L. pneumophila inhibits autophagy by injecting an effector protein called RavZ into the cytoplasm. RavZ functions as a cysteine protease and irreversibly deconjugates mammalian Atg8s from PE to inhibit autophagosome formation. Unlike Atg4 that cleaves the amide bond between terminal glycine and PE, RavZ cleaves the amide bond before glycine. As a consequence, the RavZ-cleaved Atg8 proteins cannot be relipidated, leading to inhibition of autophagy.

Next, we solved the structures of two RavZ fragments, 1–487 and 20–502. Crystal structures of the fragments are essentially identical, solved in space group I422. RavZ structures of both fragments are resolved from residues 47 to 433 and 48 to 432, respectively, whereas the missing regions at the N- and C-termini (residues 1–47 and 433–502) might be flexible and disordered. RavZ shows two major domains, the N-terminal catalytic domain (residues 49–320, catalytic triad: C258, H176, D197) and the C-terminal domain (329-423). The C-terminal domain has been recently shown to be involved in association with phosphatidylinositol 3-phsphate (PI3P) and be essential for membrane binding. Structural alignment indicated that part of the N-terminal catalytic domain of RavZ (α2–α4, β6–β9) shows a similar fold to that of the core-lipid-binding domain of Sec14, consisting of 5 β-strands and 4 α-helices (α7–α10). Similarly in RavZ, helices α2 (corresponding to α7 of Sec14) and α4 (corresponding to α8 of Sec14) along β sheets form a large hydrophobic interface. However, the hydrophobic pocket is closed in RavZ, suggesting that a conformational change may be required to accommodate the fatty acid chains. It should be noted that the LBS of RavZ is closed without showing a binding pocket for lipid, whereas a clear hydrophobic binding cavity that can accommodate fatty acid chains is observed in free Sec14 structures. Because the PE moiety involves interaction with residues located deep in the LBS fold, there must be a conformational change to open the lipid-binding site, for example, by outward movement of α4.

> GPGEQESDIDEFDLLEGDEKLPGDSELDKTTSIYPPETSWEVNKGMNSSRLHKLYSLFFDKSSAFYLGDDVSVLEDKPLTGAYGFQSKKNDQQIFLFRPDSDYVAGYHVDAKSDAGWVNDKLDRRLSEISEFCSKATQPATFILPFVEMPTDITKGVQHQVLLTISYDPKSKQLTPTVYDSIGRDTYSESLSSYFKGKYRTTCDEILTQSIEKAIKSTDFTLGKFTRAAYNHQNRLTEGNCGSYTFRTIKEVISSSAQGTEVKIPGSGYITSNSYLTSQHVQDIESCIKYRNLGVVDIESALTEGKTLPVQLSEFIVALEDYGKLRSQQSEKSMLNFIGYSKTAKLTAVELLIGILNDIKGKNEISESQYDKLVKEVDCLMDSSLGKLVQFHLKNLGAESLQKLVLPCVKFDDTIDDFVTIEKDELFDVPDITGEELASKKGIEQGALDKEALLKQKQIKTDLLDLREEDKTGLKKPLHGGIKVK>SRKTYTLTDYLKNTYRLKLYSLRWISDHEYLYKQENNILVFNAEYGNSSVFLENSTFDEFGHSI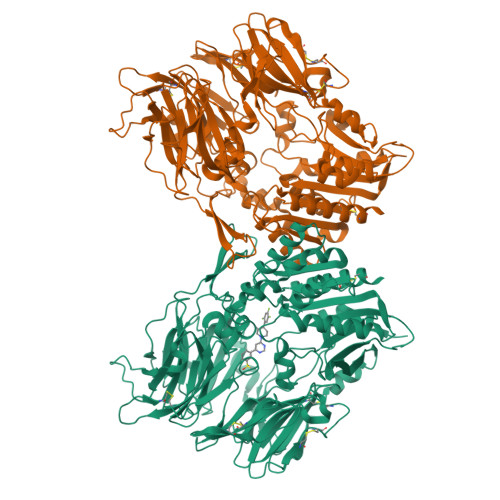NDYSISPDGQFILLEYNYVKQWRHSYTASYDIYDLNKRQLITEERIPNNTQWVTWSPVGHKLAYVWNNDIYVKIEPNLPSYRITWTGKEDIIYNGITDWVYEEEVFSAYSALWWSPNGTFLAYAQFNDTEVPLIEYSFYSDESLQYPKTVRVPYPKAGAVNPTVKFFVVNTDSLSSVTNATSIQITAPASMLIGDHYLCDVTWATQERISLQWLRRIQNYSVMDICDYDESSGRWNCLVARQHIEMSTTGWVGRFRPSEPHFTLDGNSFYKIISNEEGYRHICYFQIDKKDCTFITKGTWEVIGIEALTSDYLYYISNEYKGMPGGRNLYKIQLSDYTKVTCLSCELNPERCQYYSVSFSKEAKYYQLRCSGPGLPLYTLHSSVNDKGLRVLEDNSALDKMLQNVQMPSKKLDFIILNETKFWYQMILPPHFDKSKKYPLLLDVYAGPCSQKADTVFRLNWATYLASTENIIVASFDGRGSGYQGDKIMHAINRRLGTFEVEDQIEAARQFSKMGFVDNKRIAIWGWSYGGYVTSMVLGSGSGVFKCGIAVAPVSRWEYYDSVYTERYMGLPTPEDNLDHYRNSTVMSRAENFKQVEYLLIHGTADDNVHFQQSAQISKALVDVGVDFQAMWYTDEDHGIASSTAHQHIYTHMSHFIKQCFS[2x]>[6x]MKYAEGTRPFTILIEGNIGSGKTTYLNHFEKYKDDICLLTEPVEKWRNVNGVNLLELMYKDPKKWAMPFVSYVTLTMLQMHTQPTNKKVKI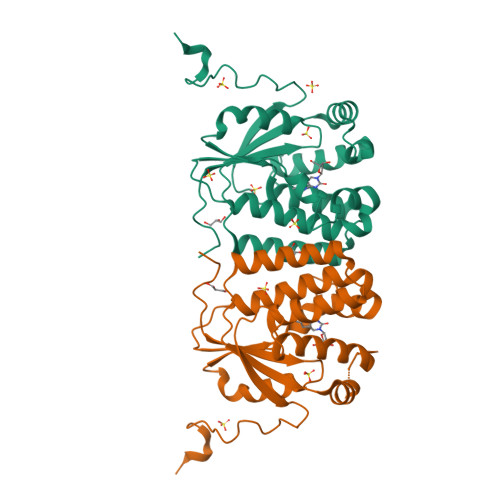MERSIFSARYCFVENMRRNGWLEQGMYNTLEEWYKFIEESIHIQADLIIYLRTSPEVAYERIRKRGRPEEKNVPLEYLQQLHQLHEDWLIHQRRPQSCKVLVLDADLNLENIGTEYQRSESSIFDAISSNQQP>[2x]ILGGREAEAHARPYMASVQLNGAHLCGGVLVAEQWVLSAAHCLEDAADGKVQVLLGAHSLSQPEPSKRLYDVLRAVPHPDSQPDTIDHD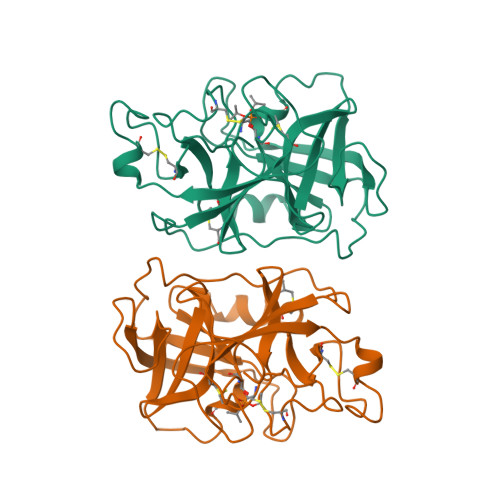LLLLQLSEKATLGPAVRPLPWQRVDRDVAPGTLCDVAGWGIVNHAGRRPDSLQHVLLPVLDRATCNRRTHHDGAITERLMCAESNRRDSCKGDSGGPLVCGGVLEGVVTSGSRVCGNRKKPGIYTRVASYAAWIDSVLA>[8x]MYNYKE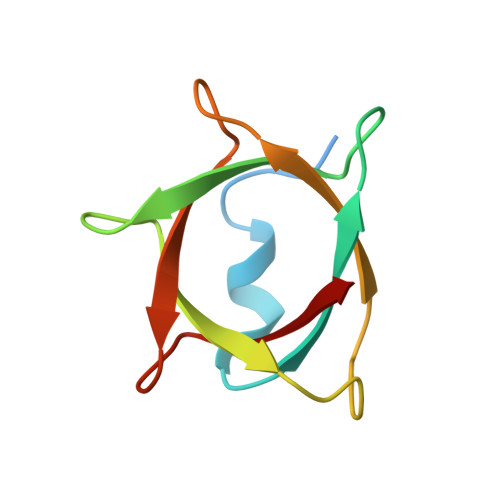VKHMGYGKGYLAMFKNKKVRFKVVNSFPDLKVQFVTSFPDYKVKISNSSSFCEETIKIQVVTSFPDVKLQKVTSFGDFEAYID>MTLTASSSSRAVTNSPVVVALDYHNRDDALAFVDKIDPRDCRLKVGKEMFTLFGPQFVRELQQRGFDIFLDLKFHDIPNTAAHAVAAAADLGVWMVNVHASGGARMMTAAREALVPFGKDAPLLIAVTVLTSM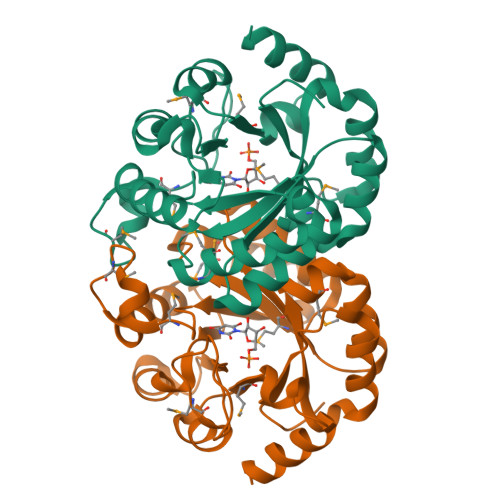EASDLVDLGMTLSPADYAERLAALTQKCGLDGVVCSAQEAVRFKQVFGQEFKLVTPGIRPQGSEAGDQRRIMTPEQALSAGVDYMVIGRPVTQSVDPAQTLKAINASLQRSA[16x]4-methyl-2-[4-(trifluoromethyl)phenyl]-1,3-thiazole-5-carboxylic 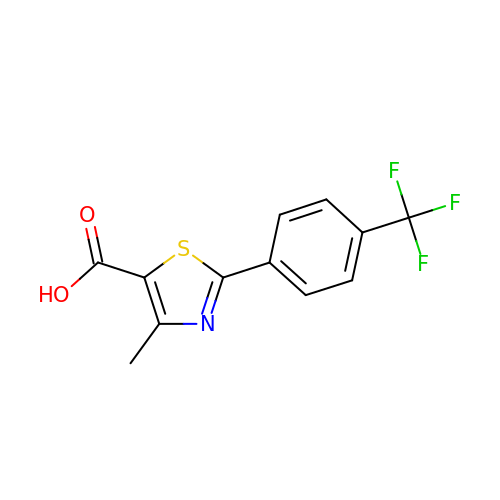acid | C12 H8 F3 N O2 S | DRFFZMPSUPHSJN-UHFFFAOYSA-N>MHHHHHHAMAQLGEMVTVLSIDGGGIRGIIPATILEFLEGQLQEMDNNADARLADYFDVIGGTSTGGLLTAMISTPNENNRPFAAAKEIVPFYFEHGPQIFNPSGQILGPKYDGKYLMQVLQEKLGETRVHQALTEVVISSFDIKTNKPVIFTKSNLANSPELDAKMYDISYSTAAAPTYFPPHYFVTNTSNGDEYEFNLVDGAVATVADPALLSISVATRLAQKDPAFASIRSLNYKKMLLLSLGTGTTSEFDKTYTAKEAATWTAVHWMLVI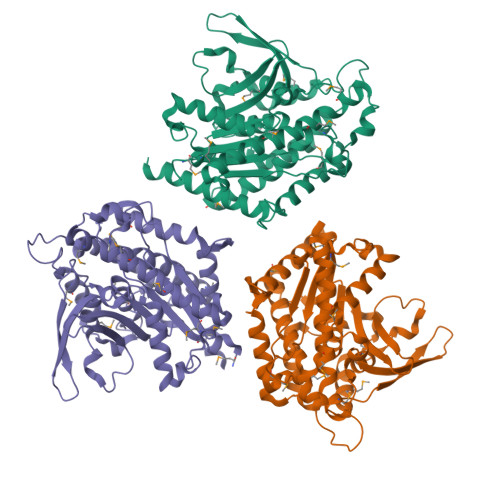QKMTDAASSYMTDYYLSTAFQALDSKNNYLRVQENALTGTTTEMDDASEANMELLVQVGENLLKKPVSEDNPETYEEALKRFAKLLSDRKKLRANKASY[3x]>ANPLYQKHIISINDLSRDDLNLVLATAAKLKANPQPELLKHKVIASCFFEASTRTRLSFETSMHRLGASVVGFSDSANTSLGKKGETLADTISVISTYVDAIVMRHPQEGAARLATEFSGNVPVLNAGDGSNQHPTQTLLDLFTIQETQGRLDNLHVAMVGDLEYGRTVHSLTQALAKFDGNRFYFIAPDALAMPQYILDMLDEKGIAWSLHSSIEEVMAEVDILYMTRVQKERLDPSKYANVKAQFVLRASDLHNAKANMKVLHPLPRVDEIATDVDKTPHAWYFQQAGNGIFARQALLALVLNRDLVL[6x];>[6x]MTHDNKLQVEAIKRGTVIDHIPAQIGFKLLSLFKLTETDQRIT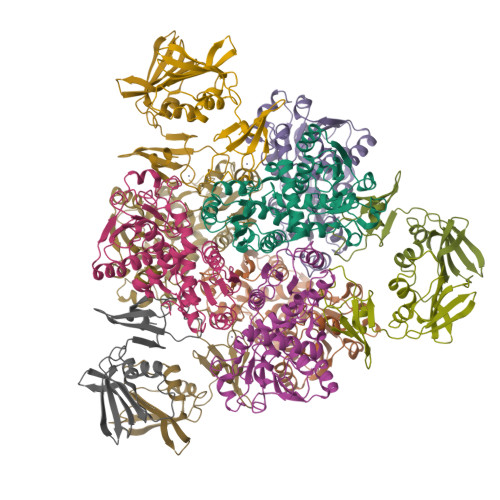IGLNLPSGEMGRKDLIKIENTFLSEDQVDQLALYAPQATVNRIDNYEVVGKSRPSLPERIDNVLVCPNSNCISHAEPVSSSFAVRKRANDIALKCKYCEKEFSHNVVLAN> MSLRSGGRRRADPGADGEASRDDGATSSVSALKRLERSQWTDKMDLRFGFERLKEPGEKTGWLINMHPTEILDEDKRLGSAVDYYFIQDDGSRFKVALPYKPYFYIATRKGCEREVSSFLSKKFQGKIAKVETVPKEDLDLPNHLVGLKRNYIRLSFHTVEDLVKVRKEISPAVKKNREQDHASDAYTALLSSVLQRGGVITDEEETSKKIADQLDNIVDMREYDVPYHIRLSIDLKIHVAHWYNVRYRGNAFPVEITRRDDLVERPDPVVLAFAIATTKLPLKFPDAETDQIMMISYMIDGQGYLITNREIVSEDIEDFEFTPKPEYEGPFCVFNEPDEAHLIQRWFEHVQETKPTIMVTYNGDFFDWPFVEARAAVHGLSMQQEIGFQKDSQGEYKAPQCIHMDCLRWVKRDSYLPVGSHNLKAAAKAKLGYDPVELDPEDMCRMATEQPQTLATYSVSDAVATYYLYMKYVHPFIFALCTIIPMEPDEVLRKGSGTLCEALLMVQAFHANIIFPNKQEQEFNKLTDDGHVLDSETYVGGHVEALESGVFRSDIPCRFRMNPAAFDFLLQRVEKTLRHALEEEEKVPVEQVTNFEEVCDEIKSKLASLKDVPSRIECPLIYHLDVGAMYPNIILTNRLQPSAMVDEATCAACDFNKPGANCQRKMAWQWRGEFMPASRSEYHRIQHQLESEKFPPLFPEGPARAFHELSREEQAKYEKRRLADYCRKAYKKIHITKVEERLTTICQRENSFYVDTVRAFRDRRYEFKGLHKVWKKKLSAAVEVGDAAEVKRCKNMEVLYDSLQLAHKCILNSFYGYVMRKGARWYSMEMAGIVCFTGANIITQARELIEQIGRPLELDTDGIWCVLPNSFPENFVFKTTNVKKPKVTISYPGAMLNIMVKEGFTNDQYQELAEPSSLTYVTRSENSIFFEVDGPYLAMILPASKEEGKKLKKRYAVFNEDGSLAELKGFEVKRRGELQLIKIFQSSVFEAFLKGSTLEEVYGSVAKVADYWLDVLYSKAANMPDSELFELISENRSMSRKLEDYGEQKSTSISTAKRLAEFLGDQMVKDAGLSCRYIISRKPEGSPVTERAIPLAIFQAEPTVRKHFLRKWLKSSSLQDFDIRAILDWDYYIERLGSAIQKIITIPAALQQVKNPVPRVKHPDWLHKKLLEKNDVYKQKKISELFTLEGRRQVTMAEASEDSPRPSAPDMEDFGLVKLPHPAAPVTVKRKRVLWESQEESQDLTPTVPWQEILGQPPALGTSQEEWLVWLRFHKKKWQLQARQRLARRKRQRLESAEGVLRPGAIRDGPATGLGSFLRRTARSILDLPWQIVQISETSQAGLFRLWALVGSDLHCIRLSIPRVFYVNQRVAKAEEGASYRKVNRVLPRSNMVYNLYEYSVPEDMYQEHINEINAELSAPDIEGVYETQVPLLFRALVHLGCVCVVNKQLVRHLSGWEAETFALEHLEMRSLAQFSYLEPGSIRHIYLYHHAQAHKALFGIFIPSQRRASVFVLDTVRTDQMPSLGALYSAEHGLLLEKVGPELLPPPKHTFEVRAETDLKTICRAIQRFLLAYKEERRGPTLIAVQSSWELKRLASEIPVLEEFPLVPICVADKINYGVLDWQRHGARRMIRHYLNLDTCLSQAFEMSRYFHIPIGNLPEDISTFGSDLFFARHLQRHNHLLWLSPTARPDLGGKEADDNCLVMEFDDQATVEINSSGCYSTVCVELDLQNLAVNTILQSHHVNDMEGADSMGISFDVIQQASLEDMITGGQAASAPASYDETALCSNTFRILKSMVVGWVKEITQYHNIYADNQVMHFYRWLRSPSSLLHDPALHRTLHNMMKKLFLQLIAEFKRLGSSVIYANFNRIILCTKKRRVEDAIAYVEYITSSIHSKETFHSLTISFSRCWEFLLWMDPSNYGGIKGKVSSRIHCGLQDSQKAGGAEDEQENEDDEEERDGEEEEEAEESNVEDLLENNWNILQFLPQAASCQNYFLMIVSAYIVAVYHCMKDGLRRSAPGSTPVRRRGASQLSQEAEGAVGALPGMITFSQDYVANELTQSFFTITQKIQKKVTGSRNSTELSEMFPVLPGSHLLLNNPALEFIKYVCKVLSLDTNITNQVNKLNRDLLRLVDVGEFSEEAQFRDPCRSYVLPEVICRSCNFCRDLDLCKDSSFSEDGAVLPQWLCSNCQAPYDSSAIEMTLVEVLQKKLMAFTLQDLVCLKCRGVKETSMPVYCTCAGDFALTIHTQVFMEQIGIFRNIAQHYGMSYLLETLEWLLQKNPQLGH;>MFEARLVQGSILKKVLEALKDLINEACWDISSSGVNLQSMDSSHVSLVQLTLRSEGFDTYRCDRNLAMGVNLTSMSKILKCAGNEDIITLRAEDNADTLALVFEAPNQEKVSDYEMKLMDLDVEQLGIPEQEYSCVVKMPSGEFARICRDLSHIGDAVVISCAKDGVKFSASGELGNGNIKLSQTSNVDKEEEAVTIEMNEPVQLTFALRYLNFFTKATPLSSTVTLSMSADVPLVVEYKIADMGHLKYYLAPKIEDEEGS[3x]

In eukaryotes, the leading strand DNA is synthesized by Polε and the lagging strand by Polδ. These replicative polymerases have higher processivity when paired with the DNA clamp PCNA. Here we report two cryo-EM structures of human Polε–PCNA–DNA complex, one in an incoming nucleotide bound state and the other in a nucleotide exchange state. The structures reveal an unexpected three-point interface between the Polε catalytic domain and PCNA, with the conserved PIP (PCNA interacting peptide)-motif, the unique P-domain, and the thumb domain each interacting with a different protomer of the PCNA trimer.

The quaternary human Polε–PCNA–DNA–dTTP structure contains the incoming dTTP that base-pairs with the template in the polymerase site and has the finger domain in the closed conformation. We refer to this structure as the “nucleotide bound state”. The high-quality map allowed us to build an atomic model for the quaternary complex. In the nucleotide bound state, the P-domain, the thumb domain, and the C-terminal PIP motif of catalytic POLE1-NTD each interact with a separate PCNA protomer. In the case of the P-domain interacting with PCNA-1 (PCNA protomer-1), the ends of two P-domain α-helices insert into the PCNA-1 PIP-binding pocket, with His-684, Arg-685, Gln-689, Tyr-726, and Lys-729 forming five hydrogen bonds (H-bonds) with PCNA-1 Asp-257, Pro-253, His-44, Lys-254, and Asp-41, respectively. In the case of the thumb domain interacting with PCNA-2 (PCNA protomer-2), two short thumb loops insert into the PCNA-2 PIP-binding pocket, with thumb residues Glu-1085 and Ser-1117 forming two H-bonds with PCNA-2 Tyr-211 and Ile-255, respectively. The PIP motif of Polε adopts a short 310 helix and inserts into the hydrophobic PIP-binding pocket of PCNA-3. The extended β-strand following the PIP motif interacts with the PCNA-3 interdomain connecting loop (IDCL) to form a two-stranded β-sheet. Inside the catalytic pocket, the incoming dTTP has well-defined EM density and forms a base-pair with an adenine of the template strand. The dTTP triphosphate inserts between the palm and finger to H-bond with the main chain nitrogen atom of Ala-629 of the palm and the finger side chains of Arg-765, Lys-769, Lys-809, and Asn-813.> GMKDNPISPTIPLDQDGVHHGFLKLPYSRDDSAWGSVMIPITVIQNGAGKTALLTGANHGDEYEGPVALQELAATTRAEDVTGRLIIVPYFNYPAFRASARTSPIDRGNLNRAFPGRPDGTVTQKIADYFQRTLLPMADVAVDFHSGGKTLDFVPFAAAHILEDKVLQDACFAAMQAFNAPYSVQLLEIDSEGMYDTAVEEMGKVLVTTELGGGGMSTARSNAIAKKGLRNVL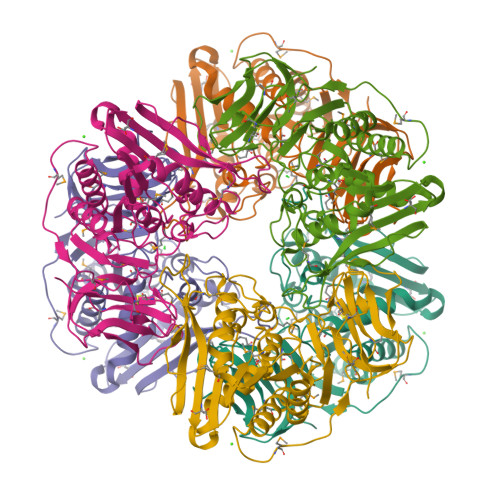IHFGILQGEMQIDPSVTLDMPDGDCYLFSEHDGLFEIMIDLGEPVQEGDLVARVWSPDRTGEAPVEYRARRSGVLISRHFPGMIKSGDCAAVIGVVEG> GCGGAUUUAGCUCAGUUGGGAGAGCGCCAGACUGAAGAUCUGGAGGUCCUGUGUUCGA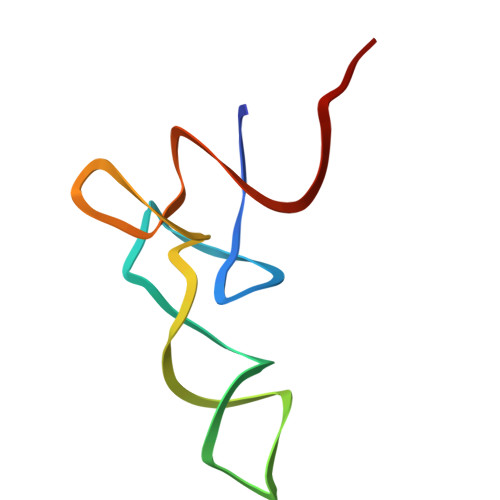UCCACAGAAUUCGCACCA>[2x]MKHHHHHHMKQNSPLDEENLTQENQDRGTHVDRGLASANVDFAFSLYKQLVLKAPDKNVIFSPLSISTALAFLSLGAHNTTLTEILKGLKFNLTETSEAEIHQSFQH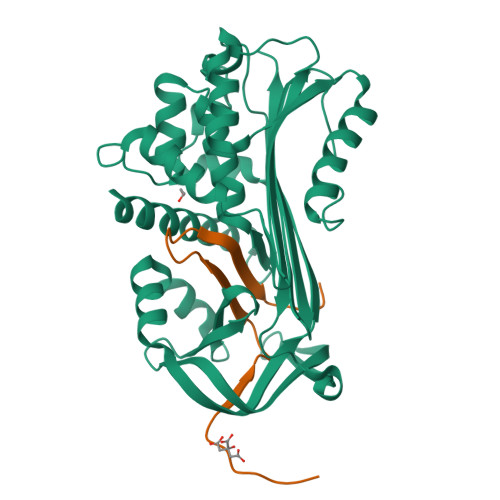LLRTLNQSSDELQLSMGNAMFVKEQLSLLDRFTEDAKRLYGSEAFATDFQDSAAAKKLINDYVKNGTRGKITDLIKDLDSQTMMVLVNYIFFKAKFEMPFDPQDTHQSRFYLSKKKYVMVPMMSLHHLTIPYFRDEELSCTVVQLNYTGNASALFILPDQDKMEEVEAMLSQETLSRFFDSLEFREIGELYLPKFSISRDYNLNDILLQLGIEEAFTSKADLSGITGARNLAVSQVVHKAVLDVFEEGTERSAATALKGPRQ;>ITAVETRTIVRFNRPFLMIIVDHFTWSIFFMSKVTNPKQA[2x]>MGYVGIKIRLTDVAPQAQELFKKESLDVKENKVYLVAATLRPETMYGQTCCFVSPKIDYGVFDAGNGDYFITTERAFKNMSFQNLTPKRGYYKPLFTINGKTLIGSRIDAPYAVNKNLRVLPMETVLATKGTGVVTCVPSDSPDDFVTTRDLANKPEYYGIEKDWVQTDIVPIVHTEKYGDKCAEFLVNDLKIQSPKDSVQLANAKELAYKEGFYNGTML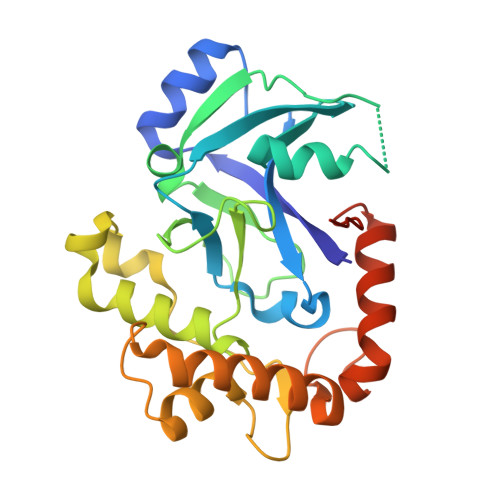IGKYKGDKVEDAKPKVKQDLIDEGLAFVYNEPELEHHHHHH[4x]>DNSYKMDYPEMGL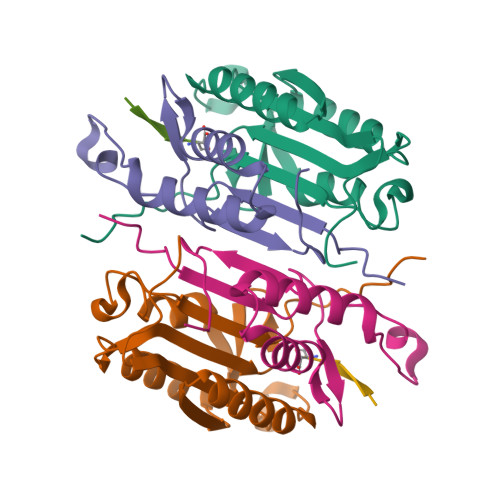CIIINNKNFHKSTGMTSRSGTDVDAANLRETFRNLKYEVRNKNDLTREEIVELMRDVSKEDHSKRSSFVCVLLSHGEEGIIFGTNGPVDLKKITNFFRGDRCRSLTGKPKLFIIQACRGTELDCGIET[2x];>[2x]CHKIPVEADFLYAYSTAPGYYSWRNSKDGSWFIQSLCAMLKQYADKLEFMHILTRVNRKVATEFESFSFDATFHAKKQIPCIVSMLTKELYFYHH;>[2x]XVDKVD> A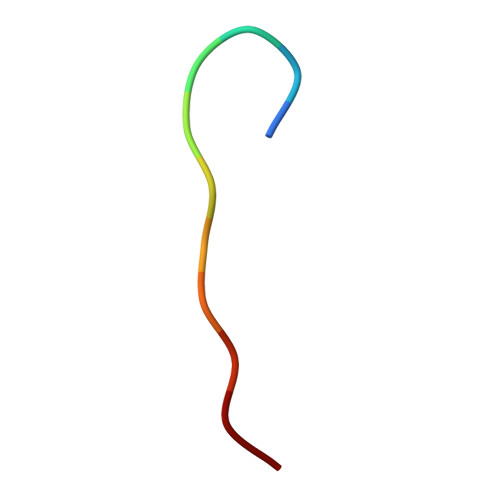AAAAAAAAAA>MWSHPQFEKENLYFQGSMDDISPSELKTILHSKRANLYYLQHCRVLVNGGRVEYVTDEGRHSHYWNIPIANTTSLLLGTGTSITQAAMRELARAGVLVGFCGGGGTPLFSANEVDVEVSWLTPQSEYRPTEYLQRWVGFWFDEEKRLVAARHFQRARLERIRHSWLEDRVLRDAGFAVDATALAVAVEDSARALEQAPNHEHLLTEEARLSKRLFKLAAQATRYGEFVRAKRGSGGDPANRFLDHGNYLAYGLAATATWVLGIPHGLAVLHGKTRRGGLVFDVADLIKDSLILPQAFLSAMRGDEEQDFRQACLDNLSRAQALDFMIDTLKDVAQRSTVSA[4x];>GPMGALTKAEIAERLYEELGLNKREAKELVELFFEEIRQALEHNEQVKLSGFGNFDLRDKRQRPGRNPKTGEEIPITARRVVTFRPGQKLKARVEAYAGTKS[2x];>GPMTKSELIERIVTHQGQLSAKDVELAIKTMLEQMSQALATGDRIEIRGFGSFSLHYRAPRVGRNPKTGESVRLDGKFVPHFKPGKELRDRVNEPE[2x];>MNILLVSQCEKRALSETRRILDQFAERRGERTWQTPITQAGLDTLRRLLKKSARRNTAVACHWIRGRDHSELLWIVGDASRFNAQGAVPTNRTCRDILRKEDENDWHSAEDIRLLTVMAALFHDIGKASQAFQAKLRNRGKPMADAYRHEWVSLRLFEAFVGPGSSDEDWLRRLADKRETGDAWLSQLARDDRQSAPPGPFQKSRLPPLAQAVGWLIVSHHRLPNGDHRGSASLARLPAPIQSQWCGARDADAKEKAACWQFPHGLPFASAHWRARTALCAQSMLERPGLLARGPALLHDSYVMHVSRLILMLADHHYSSLPADSRLGDPNFPLHANTDRDSGKLKQRLDEHLLGVALHSRKLAGTLPRLERQLPRLARHKGFTRRVEQPRFRWQDKAYDCAMACREQAMEHGFFGLNLASTGCGKTLANGRILYALADPQRGARFSIALGLRSLTLQTGQAYRERLGLGDDDLAILVGGSAARELFEKQQERLERSGSE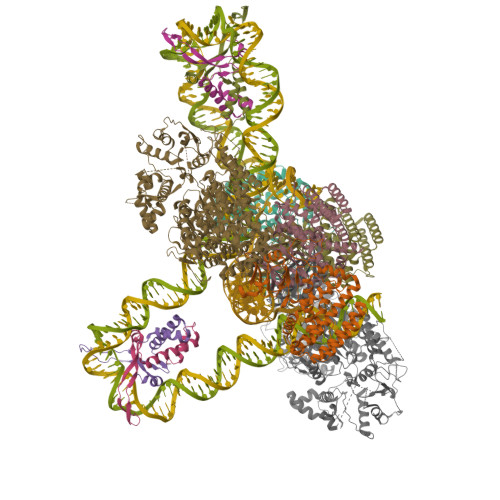SAQELLAENSHVHFAGTLEDGPLREWLGRNSAGNRLLQAPILACTIDHLMPASESLRGGHQIAPLLRLMTSDLVLDEVDDFDIDDLPALSRLVHWAGLFGSRVLLSSATLPPALVQGLFEAYRSGREIFQRHRGAPGRATEIRCAWFDEFSSQSSAHGAVTSFSEAHATFVAQRLAKLEQLPPRRQAQLCTVHAAGEARPALCRELAGQMNTWMADLHRCHHTEHQGRRISFGLLRLANIEPLIELAQAILAQGAPEGLHVHLCVYHSRHPLLVRSAIERQLDELLKRSDDDAAALFARPTLAKALQASTERDHLFVVLASPVAEVGRDHDYDWAIVEPSSMRSIIQLAGRIRRHRSGFSGEANLYLLSRNIRSLEGQNPAFQRPGFETPDFPLDSHDLHDLLDPALLARIDASPRIVEPFPLFPRSRLVDLEHRRLRALMLADDPPSSLLGVPLWWQTPASLSGALQTSQPFRAGAKERCYALLPDEDDEERLHFSRYEEGTWSNQDNLLRNLDLTYGPRIQTWGTVNYREELVAMAGREDLDLRQCAMRYGEVRLRENTQGWSYHPYLGFKKYN[2x]> MSKREETGLATSAGLIRYMDETFSKIRVKP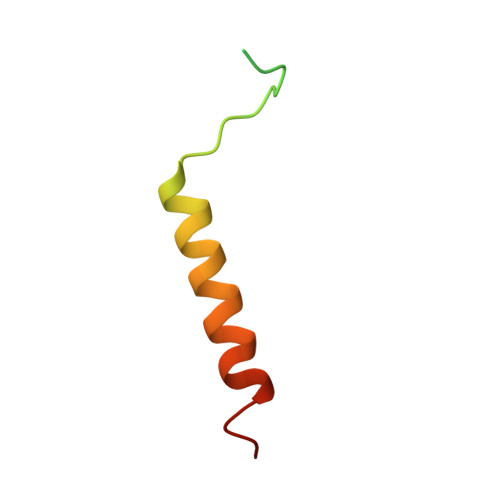EHVIGVTVAFVIIEAILTYGRFL> MSSHHHHHHMQFDVTIEIPKGQRNKYEVDH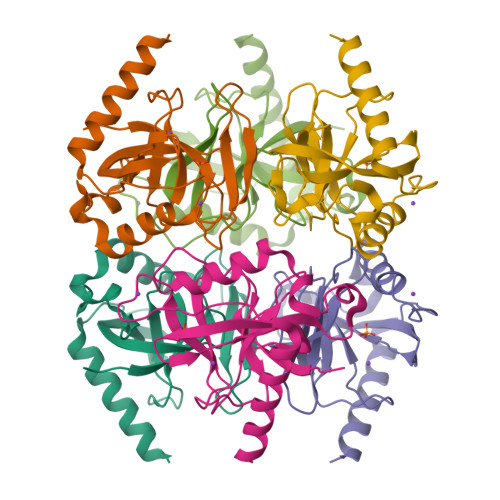ETGRVRLDRYLYTPMAYPTDYGFIEDTLGDDGDPLDALVLLPQPVFPGVLVAARPVGMFRMVDEHGGDDKVLCVPAGDPRWDHVQDIGDVPAFELDAIKHFFVHYKDLEPGKFVKAADWVDRAEAEAEVQRSVERFKAGTH> GSHMGTRDDEYDYLFKVVLIGDSGVGKSNLLSRFTRNEFNLESKSTIGVEFATRSIQVDGKTIKAQIWDTAGLERYRAITSAYYRGAVGALLVY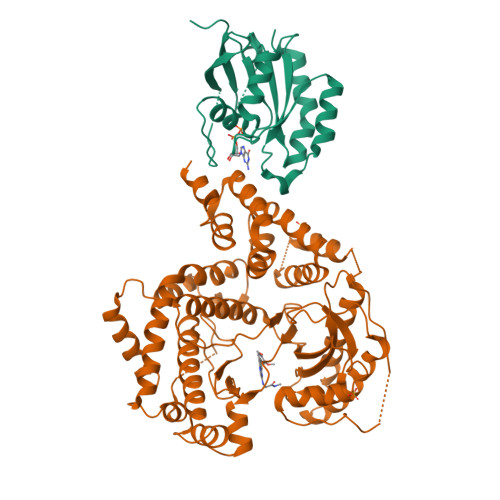DIAKHLTYENVERWLKELRDHADSNIVIMLVGNKSDLRHLRAVPTDEARAFAEKNGLSFIETSALDSTNVEAAFQTILTEIYRIVSQKQMSDRRENDMSPSNNVVPIHVPPTTENKPKVQCCQNI;> GSHMQNNSAKQSWLLRLFESKLFDISMAISYLYNSKEPGVQAYIGNRLFCFRNEDVDFYLPQLLNMYIHMDEDVGDAIKPYIVHRCRQSINFSLQCALLLGAYSSDMHISTQRHSRGTKLRKLILSDELKPANLKRTAANPKVENEDEPVRLAPEREFIKSLMAIGKRLATLPTKEQKTQRLISELSLLNHKLPARVWLPTAGFDHHVVRVPHTQAVVLNSKDKAPYLIYVEVLECENFDTTSVPARIPENRRDPEDPSAVALKEPWQEKVRRIREGSPYGHLPNWRLLSVIVKCGDDLRQELLAFQVLKQLQSIWEQERVPLWIKPYKILVISADSGMIEPVVNAVSIHQVKKQSQLSLLDYFLQEHGSYTTEAFLSAQRNFVQSCAGYCLVCYLLQVKDRHNGNILLDAEGHIIHIDFGFILSSSPRNLGFETSAFKLTTEFVDVMGGLDGDMFNYYKMLMLQGLIAARKHMDKVVQIVEIMQQGSQLPCFHGSSTIRNLKERFHMSMTEEQLQLLVEQMVDGSMRS> MSVEVYRQKIEKG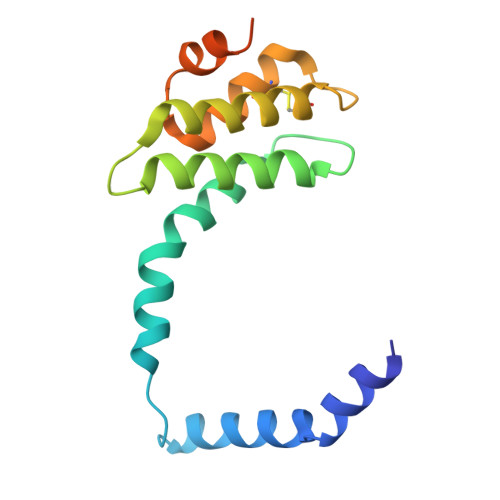GYSAAYEATRRYEREEIEVLSWSSRWESAWSKFGEAVKALGKIEGAPRALVIAKVQEALAYMSKPLPNMKLAMAAAVQAVRACEQLPGMNRERCLDAVAGALGVAKDWIRREMTGGGGGGGGGGGGGGGAVV5-methyl-1-[1-[(6-phenoxypyridin-2-yl)methyl]piperidin-4-yl]pyrimidine-2,4-dione | C22 H24 N4 O3 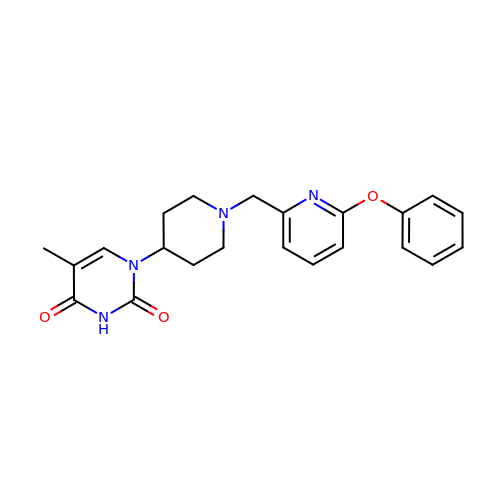| BKRRWLAIGUKKJX-UHFFFAOYSA-N In this research, using protein-RNA crystal structures, we demonstrate that multiple structural determinants collaborate to establish the dual enzymatic activities of RlmCD, which has been previously shown to catalyze C5 methylation at both U747 and U1939 of 23S rRNA in some gram-positive bacteria. However, in S. pneumoniae and Bacillus subtilis, which both belong to gram-positive bacteria, RlmCD and its homologue YefA have been proven to be dual-functional methyltransferases to catalyze both m5U747 and m5U1939 in 23S rRNA. We previously determined the crystal structure of apo-form RlmCD, which highly resembles that of RumA and contains three individual domains, including the N-terminal TRAM domain, central domain, and C-terminal catalytic domain. In all structures, the cofactors were modeled as SAH, due to the missing electron density of the methyl group, while its density was clearly observed attaching to the base C5 atom of U747 or U1939, indicating that the complexes gained in the crystal structures all exist as the trapped enolate intermediate 3, given that E443Q eliminates the final step of proton abstraction from C5.

A similar RNA design was also applied to co-crystalize the RlmCD with SAM and an 8-nt U1939-containing RNA stretches (5′-1936AAAUUCCU1943-3′, U1939L) to understand the mutual recognition between RlmCD and U1939 site on 23S rRNA. Interestingly, in the RlmCD-SAH-U1939L complex structure, the U1939-containing RNA substrate also adopts a very similar conformation to that of U747L, even though their sequences are totally different, suggesting that both RNAs were re-shaped by the catalytic groove of RlmCD to adopt an optimal conformation for protein-RNA recognition and subsequent catalysis reaction. The nucleotide base-flipping was also observed for U1939 in the RlmCD-SAH-U1939L structure. Compared with U747, U1939 in the structure of RlmCD-SAH-U1939L exhibits a totally identical interaction mode with RlmCD, suggesting that the catalytic mechanism RlmCD employed for two different RNA substrates are quite similar. As the corresponding nucleotide to G748 in U1939L, however, U1940 maintains only one hydrogen bond with the main chain hydroxyl group of Q131 using its base, while the Q131 main chain is also involved in two additional hydrogen bonds with the bases of C1941 and C1942, respectively. N249, whose side-chain originally makes multiple hydrogen bonds with the bases of three different nucleotides in the RlmCD-SAH-U747L structure, forms only one side-chain-to-base hydrogen bond with A1937. The most striking difference between the two complex structures of RlmCD is that the aromatic side-chain of F145 in RlmCD-SAH-U1939L swings away from its position in RlmCD-SAH-U747L by an angle of ~135°, without disturbing the base-stacking between U1940 and C1941. In addition, the side-chain of F146 also shifts by ~1.4 Å away from RNA nucleotide.

> MLKKNDIVEVEIVDLTHEGAGVAKVDGLVFFVENALPSEKILMRVLKVNKKIGFGKVEKYLVQSPHRNQDLDLAYLRSGIADLGHLSYPEQLKFKTKQVKDSLYKIAGIADVEVAETLGMEHPVKYRNKAQVPVRRVNGVLETGFFRKNSHNLMPLEDFFIQDPVIDQVVVALRDLLRRFDLKPYDEKEQSGLIRNLVVRRGHYSGQIMVVLVTTRPKVFRVDQLIEQVIKQFPEIVSVMQNINDQNTNAIFGKEWRTLYGQDYITDQMLGNDFQIAGPAFYQVNTEMAEKLYQTAIDFAELKKDDVIIDAYSGIGTIGLSVAKHVKEVYGVELIPEAVENSQKNASLNKITNAHYVCDTAENAMKKWLKEGIQPTVILVDPPRKGLTESFIKASAQTGADRIAYISCNVATMARDIKLYQELGYELKKVQPVDLFPQTHHVQTVALLSKLD1-ethyl-3-{4-[(E)-2-(pyridin-3-yl)ethenyl]-5-(1H-pyrrol-2-yl)-1,3-thiazol-2-yl}urea 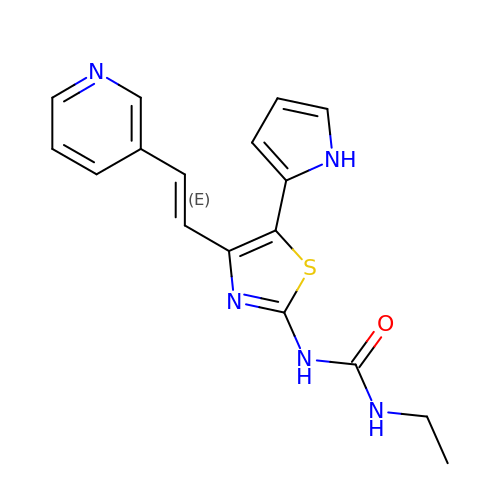| C17 H17 N5 O S | KXSSNSOHTLLWNT-BQYQJAHWSA-N> PISPIETVPVKLKPGMDGPKVKQWPLTEEKIKALVEICTEMEKEGKISKIGPENPYNTPVFAIKKKDSTKWRKLVDFRELNKRTQDFWEVQLGIPHPAGLKKKKSVTVLDVGDAYFSVPLDEDFRKYTAFTIPSINNETPGIRYQYNVLPQG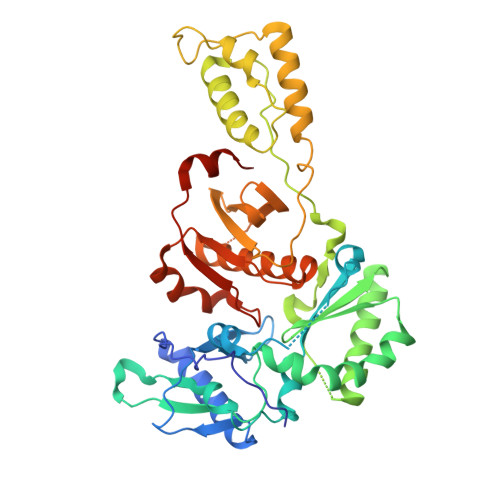WKGSPAIFQSSMTKILEPFRKQNPDIVIYQYMDDLYVGSDLEIGQHRTKIEELRQHLLRWGLYTPDKKHQKEPPFLWMGYELHPDKWTVQPIVLPEKDSWTVNDIQKLVGKLNWASQIYPGIKVRQLCKLLRGTKALTEVIPLTEEAELELAENREILKEPVHGVYYDPSKDLIAEIQKQGQGQWTYQIYQEPFKNLKTGKYARMRGAHTNDVKQLTEAVQKITTESIVIWGKTPKFKLPIQKETWETWWTEYWQATWIPEWEFVNTPPLVKLWYQLEKEPIVGAETF>GPLGSMAEAFTREDYVFMAQLNENAERYDEMVETMRKISGMEGELSDKE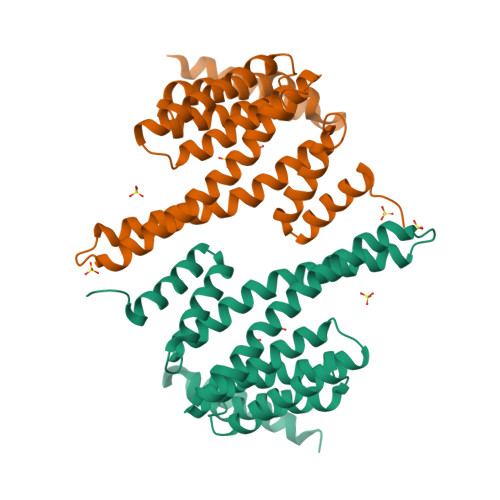RNLLSVAYKNVIGPRRAAWRIVSSIEAKEKGRQKPNAKRIEQIRVYRQKIEKELSDICNDILKLLQEQFVPRSTNADAKVFYYKMQGDYYRYLAEYSSGEDKEKIAGSALNAYNSAFEISQQLPPTHPIRLGLALNFSVFYYEILASPDRACELARKAFDAAITDLDKLTEESYKDSTLIMQLLRDNLNLWVTDSAGDDNAEEK[4x]>SNADSVELNISAAASLKEAMAKIEEEYKKVDSNVKLTVNYGASGSLQQQIEQGAPCDLFISAGQKQMKVLDEEKLLVSDTMKDLVKNDLVLISSADSSVSGMKDLTTDKVKKIAVGEAESVPAGKYADEVLTNLNLKDKLKDKLVFAKDVKEV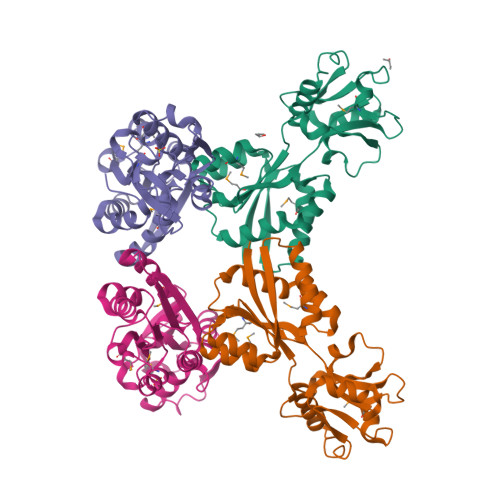LAWVQSGNADVGFVYFSDTVNNDKIKVVEKTDEKTHSPITYPVSVIKASKNVDAAKKFEEFLLSESGQKIFEEFGYKKVE[4x]Template-independent terminal ribonucleotide transferases (TENTs) catalyze the addition of nucleotide monophosphates to the 3′-end of RNA molecules regulating their fate. TENTs include poly(U) polymerases (PUPs) with a subgroup of 3′ CUCU-tagging enzymes, such as CutA in Aspergillus nidulans. CutA preferentially incorporates cytosines, processively polymerizes only adenosines and does not incorporate or extend guanosines. Here, we report structures of the catalytic core of T. terrestris CutA (TtCutA) in the apo form and its complexes with a non-hydrolyzable CTP analog and A3 RNA.

We first obtained crystals of CutA in complex with a non-hydrolyzable CTP analogue (CMPCPP). The structure was solved by molecular replacement using the apo structure and refined to 1.45 Å resolution with an Rfree of 18.1%. In the CutA-CMPCPP structure, one Ca2+ ion was observed, coordinated by side chains of both aspartates, and non-bridging oxygens of all three phosphates of the incoming nucleotide. It corresponds to metal ion B in the canonical two-metal ion mechanism of polymerases. However, it was not visible in our electron density maps and most likely absent because of the chemical modification of CMPCPP. The contacts that stabilize the incoming nucleotide in the CutA-CMPCPP structure include binding of the γ phosphate by Lys425, Ser328 and Ser444. The side chain of Tyr445 is located between the ribose ring and base of the incoming nucleotide, stabilizing it through van der Waals interactions. The 2′-OH group of the nucleotide forms a network of hydrogen bonds with Asn403 and Thr404 side chains, thus ensuring preference for incoming ribonucleotides over deoxyribonucleotides. The strongest contact may be the hydrogen bond between the O2 carbonyl of the base and side chain of Asn403. Moreover, Arg557 is located 3.3 Å from 4-NH2 of the cytosine, potentially forming a weak polar interaction.

> ETAIPFSRRRMPYSLGTDKLEKVDPDKIKSKLSEDVERKLETDMRELYDRLLPTEAIEVNRRELVSKLERLFNTEWPGHDIRVHLFGSSGNLLCSDDSDVDICITTPWRELESVCMIAELLDRHGMEKVVCVSSAKVPIVKIWDPELKLACDMNVNNTLALENTRMVRTYVSIDDRVRPLAMIIKYWTRRRVVNDAAFGGTLSSYTWICMIIAFLQLRDPPVLPALHQQHDLKLVKQDGALSDFADDIPKLRGFGAKNKDSLAVLLFQFFRFYAHEFDYDKYTLSIRMGTLLTKAEKNWQYLVNNALCVEEPFNDGRNLGNTADETSFRGLHMELRRAFDLIAEGKLEECCEQYVFPKEEERV We report the structure of tDGC from Thermotoga maritima, an important enzyme for the large scale enzymatic synthesis of c-di-GMP and the first GGDEF domain from a hyperthermophile. We expressed and crystallized a domain of the TM1788 protein from Thermotoga maritima (248 residues, WP_010865403) spanning residues 82–248, hereafter named tDGC. Cellular levels of c-di-GMP are tightly regulated by the opposing activities of diguanylate cyclases (DGCs) that synthesize c-di-GMP from two GTP molecules and phosphodiesterases (PDEs) that hydrolyze c-di-GMP into 5′-phosphoguanylyl- (3′-5′) - guanosine (pGpG) and GMP. C-di-GMP synthesis from two separate GTP molecules requires dimerization of two active GGDEF domains, with the loops bearing the GGDEF motifs of each monomer brought in close proximity to initiate the cyclization reaction.

Enzyme assays showed that tDGC is active even after days of incubation at 30°C but with very low product production, irrespective of substrate concentration, due to feedback inhibition. However, a mutation (R158A) at the I-site of tDGC significantly alleviates production inhibition, enabling synthesis of several hundred milligrams of c-di-GMP with just 10 mg of the mutant enzyme. We also report the structure of the R158A mutant of tDGC. The R158A mutation in the I-site abolishes feedback inhibition by preventing formation of the inactive c-di-GMP-locked dimer.

>MDPLTGLPNRRYFFELGNRYLDLAKREGKKVFVLFVDLAGFKAINDTYGHLSGDEVLKTVSKRILDRVARSDVVARYGGDEFTILLYDMKEEYLKSLLERILSTFREPVRVENKHLSVTPNIGVARFPEDGENLEELLKVADMRMYKAKEMKVPYFSLSLEHHHHHH[6x]>GSLIGLMKDAFQPHHHHHHHLSPHPPG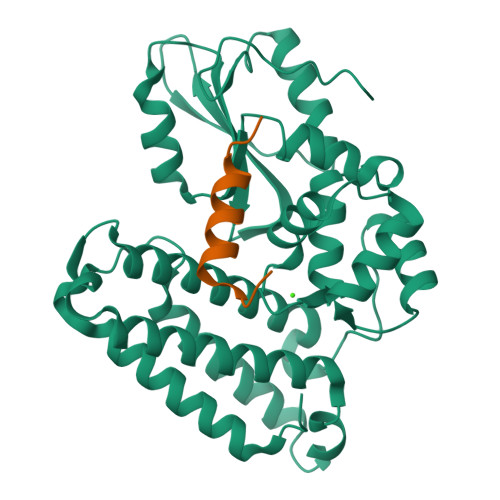TVDKKMVEKCWKLMDKVVRLCQNPKLALKNSPPYILDLLPDTYQHLRTILSRYEGKMETLGENEYFRVFMENLMKKTKQTISLFKEGKERMYEENSQPRRNLTKLSLIFSHMLAELKGIFPSGLFQGDTFRITKADAAEFWRKAFGEKTIVPWKSFRQALHEVHPISSGLEAMALKSTIDLTCNDYISVFEFDIFTRLFQPWSSLLRNWNSLAVTHPGYMAFLTYDEVKARLQKFIHKPGSYIFRLSCTRLGQWAIGYVTADGNILQTIPHNKPLFQALIDGFREGFYLFPDGRNQNPDLTGLCEPTP[2x];>[2x]LSEGLRESLSSYISLAEDP Type II DNA topoisomerases are essential enzymes that catalyze topological rearrangement of double-stranded DNA (dsDNA) to maintain chromosomes in an appropriate state. In particular, DNA gyrase introduces negative supercoils into covalently closed dsDNA molecules using the free energy generated by ATP hydrolysis. The GyrB subunit is comprised of three domains: the N-terminal ATPase domain (GHKL family), the transducer domain, and the C-terminal TOPRIM domain. Here we report the structures of bacterial GyrB43 in complex with (i) the pre-hydrolysis analog ADP⋅BeF3, (ii) the post-hydrolysis ADP⋅Pi and (iii) the product ADP.

Structures of type II topoisomerases have been determined previously for archael topoVI-B' in complex with various nucleotides and for human topoII (htopoII) in complex with AMPPNP and ADP, highlighting some of the structural changes occurring along the ATP hydrolysis pathway. In contrast, human topoisomerase II shows a semi-open ADP complex characterized by an 8° outward rotation of the transducer domain when compared with its restrained/closed AMPPNP conformation. Thus, the structure apparently represents an ADP⋅SO4 mimic of the post-hydrolysis state and the domain rotation may well be of functional relevance (see also below). Interestingly, also human topoII may undergo a similar structural transition as inferred by the comparison of the respective AMPPNP and ADP⋅SO4 complexes. As for bacterial gyrase, the pivot of the motion is at the center of the interface between the C-terminal ATPase domain helix and the transducer β-sheet, but the direction of the rotation axis is different.

>SVERIYQKKTQLEHILLRPDTYIGSVELVTQQMWVYDEDVGINYREVTFVPGLYKIFDEILVNAADNKQRDPKMSCIRVTIDPENNLISIWNNGKGIPVVEHKVEKMYVPALIFGQLLTSSNYDDDEKKVTGGRNGYGAKLCNIFSTKFTVETASREYKKMFKQTWMDNMGRAGEMELKPFNGEDYTCITFQPDLSKFKMQSLDKDIVALMVRRAYDIAGSTKDVKVFLNGNKLPVKGFRSYVDMYLKDKLDETGNSLKVIHEQVNHRWEVCLTMSEKGFQQISFVNSIATSKGGRHVDYVADQIVTKLVDVVKKKNKGGVAVKAHQVKNHMWIFVNALIENPTFDSQTKENMTLQPKSFGSTCQLSEKFIKAAIGCGIVESILNWVKFKAQVQLNKKCS[4x]D-cysteine (D-Cys) moieties are found in firefly luciferin, semisynthetic cephalosporin MT141 and malformin A. D-cysteine desulfhydrase (DCyD) is suggested to take part in the catabolic degradation of D-Cys and D-Cys-containing toxic compounds. The polypeptide fold of StDCyD is similar to those of other fold type II PLP-dependent enzymes and consists of a small domain (residues 48–161) and a large domain (residues 1–47 and 162–328). As in other PLP-dependent fold type II enzymes, the active site is situated in a large crevice between the two domains. StDCyD is specific for D-Cys and βCDA, and shows no activity with ACC, although it shares significant sequence identity with ACCDs.

Significant activity was also observed with βCDA (Km = 0.84±0.30 mM, Vmax = 173.4±82.1 µmol pyruvate produced/min/mg of protein). The crystals of StDCyD obtained in the presence of D-Cys and βCDA show the product pyruvate at a site ∼5 Å away from the substrate binding pocket. The additional electron density observed in the complex is consistent with two different binding sites for the substrate. One of these coincides with the canonical active site of fold type II enzymes and the other is 4.0–6.0 Å away from this site. The electron density observed at the active site pocket was not adequate to model the ligand used for soaking the crystals. The density could be modeled as a sulphate and two water molecules. The density at the other site 4.0–6.0 Å away from the active site could be modeled either as product of the catalytic reaction, pyruvate or final intermediate of the reaction, aminoacrylate. Examination of the residual electron density after refinement with various occupancies for pyruvate and the aminoacrylate suggested that it is more likely to represent a pyruvate. The modeled pyruvate is held by hydrogen bonding with Arg222 and Ser221.

>MRGSHHHHHHGMASMPLHHLTRFPRLEFIGAPTPLEYLPRLSDYLGREIYIKRDDVTPIAMGGNKLRKLEFLVADALREGADTLITAGAIQSNHVRQTAAVAAKLGLHCVALLENPIGTTAENYLTNGNRLLLDLFNTQIEMCDALTDPDAQLQTLATRIEAQGFRPYVIPVGGSSALGAMGYVESALEIAQQCEEVVGLSSVVVASGSAGTHAGLAVGLEHLMPDVELIGVTVSRSVAEQKPKVIALQQAIAGQLALTATADIHLWDDYFAPGYGVPNDAGMEAVKLLASLEGVLLDPVYTGKAMAGLIDGISQKRFNDDGPILFIHTGGAPALFAYHPHV[4x]> GPMDTPENVLQMLEAHMQSYKGNDPLGEWERYIQWVEENFPENKEYLITLLEHLMKEFLDK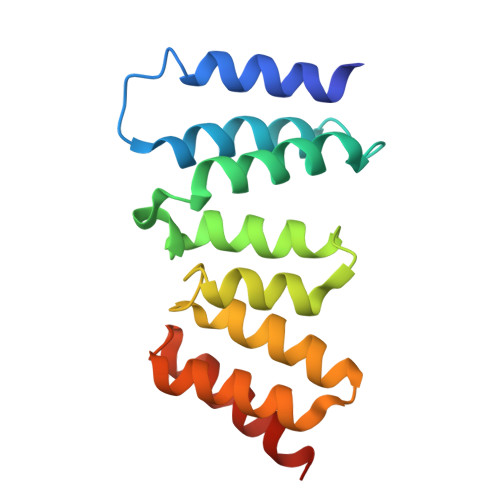KKYHNDPRFISYCLKFAEYNSDLHQFFEFLYNHGIGTLSSPLYIAWAGHLEAQGELQHASAVLQRGIQNQAEPREFLQQQYRLFQTRLTET> GAMATPWRNPAEEREKLAYRKQNMDDIDEEDDDLVGVSVRPKVPLRTMSYK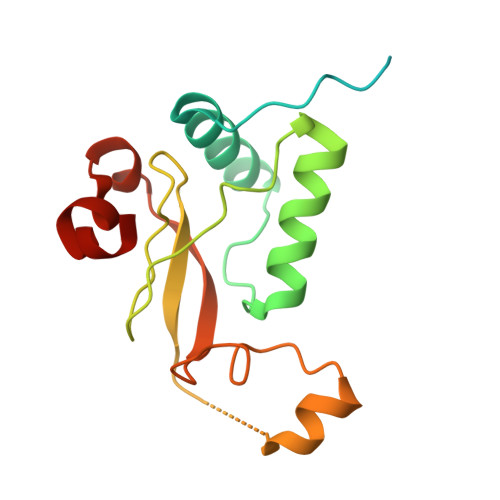LAIDMSHFIKEKGGLEGIYYSARRHRILDIYLEKEEGIIPDWQDYTSGPGIRYPKTFGWLWKLVPVNVSDEAQEDEEHYLMHPAQTSQWDDPWGEVLAWKFDPTLAYTYEAYVRYPEEFGS>[2x]MAPTRVNDGVDADEVTFVNRFTVHGAPAEFESVFARTAAFFARQPGFVRHTLLRERDKDNSYVN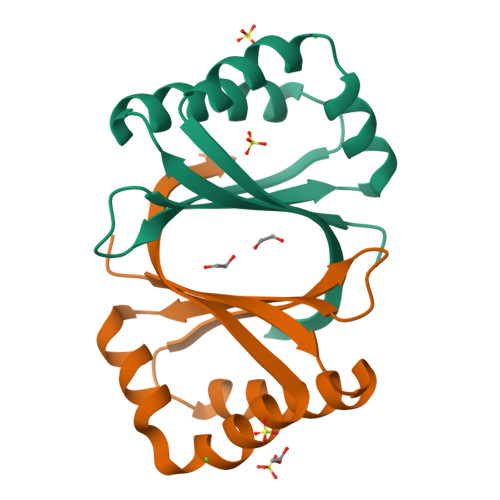IAVWTDHDAFRRALAQPGFLPHATALRALSTSEHGLFTARQTLPEGGDTTGSGHRHHHHHH>[4x]MASGMIVTDAGADQPIVFVNRAFSTITGYAPNEVLGRNARFLQGPQTDAATVARLREAIAAARPIQERILNYRKDGQPFWNQLSISPVRDETGNVVAFVGVKTDVTAHHHHHH

Flavin-binding fluorescent proteins (FbFPs), engineered from prokaryotic and eukaryotic light, oxygen, voltage (LOV) photoreceptors, are promising fluorescent reporter proteins. Their small size (about 10 kDa for monomeric FbFPs such as the improved LOV (iLOV) protein derived from Arabidopsis thaliana phototropin photoreceptors) and their oxygen-independent fluorescence make them ideal reporters to monitor transport and anaerobic biological processes. In contrast to GFP-like fluorescent reporter proteins, whose absorption and fluorescence maxima can be tuned by exchanging certain chromophore-constituting amino acids, the absorption and fluorescence of FbFPs and other flavoproteins depends on noncovalently bound flavins, whose structure cannot be influenced by mutation. Using spectroscopy, X-ray crystallography, and quantum mechanics molecular mechanics calculations, we provide a firm structural and functional understanding of spectral tuning in FbFPs.

To verify the transferability of the blue-shifting Q489K mutation, identified for the plant FbFP iLOV, we introduced the corresponding Q148K mutation into the recently presented thermostable CagFbFP protein from thermophilic phototrophic bacterium Chloroflexus aggregans. Much like iLOV–Q489K, CagFbFP–Q148K possesses a blue-shifted S0→S1 absorption band with a maximum at around 444 nm (≈3 nm blue-shifted relative to parental CagFbFP) and a blue-shifted fluorescence-emission maximum (≈6 nm blue shift relative to parental CagFbFP; compare the gray dashed line and solid blue line). To verify that the structural changes, which we observed for iLOV–Q489K, are indeed a consequence of the introduced Q489K mutation and are not due to the observed succinimide modification, we obtained the structure of the corresponding CagFbFP–Q148K variant. Altogether, we were able to obtain three types of CagFbFP–Q148K crystals, all using the precipitant solutions with pH of 6.5 (data and refinement statistics are summarized in Table S1). Interestingly, the protein also crystallized using another precipitant solution for which we obtained crystals in two crystal forms. In all of the obtained models, the C terminus of the protein is clearly unlatched, and the side chain of the introduced lysine is facing away from FMN as was found in iLOV–Q489K. Thus, the succinimide modification present in iLOV–Q489K does not influence the backbone and the conformation of the introduced Lys because this modification is absent in all CagFbFP–Q148K structures. Therefore, we conclude that irrespective of the buffer and post-translational modification, the C terminus of the iLOV–Q489K and CagFbFP–Q148K variants is unlatched, the LOV core domain is opened up to allow solvent ingress, and the introduced lysine occupies an extended conformation facing away from the FMN chromophore. The photophysical properties of the CagFbFP variants are relatively straightforward to interpret.>[2x]MFRTEDQSALRVGTDGIYPPHSFHAQDGRGELTGFDIDLIKEVAHRLNLKVE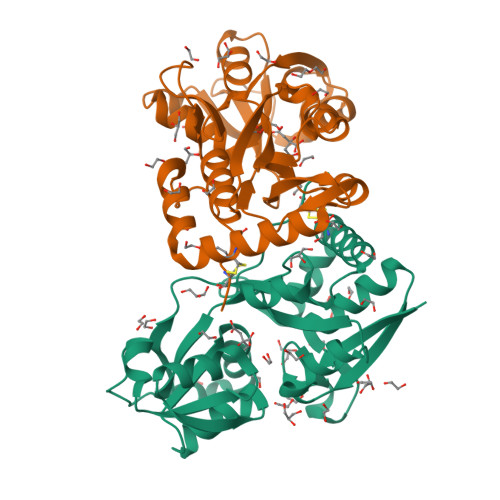FFETAVSGLITGLDTNRYDVLVNVAITPERQKKYDFSIPYIAHRVLLVVRSDQQDIRSFKDLTDKTVAQILGTDLSRFAKELKSHLVFSHNFEQSLQLLLSKRTDATMIPDIPFFNFLERRPHDGNLFKIADRMKDNSAVAFMMRKGNNKLTRSINEILCAIHLDGTYKKIFDRYFDKNIISSVPGCSS> MAQYYPGTTKVAQNRRNFCNPEYELEKLREISDEDVVKILGHRAPGEEYPSVHPPLEEMDEPEDAIREMVEPIDGAKAGDRVRYIQFTDSMYFAPAQPYVRSRAYLCRYRGADAGTLSGRQIIETRERDLEKIS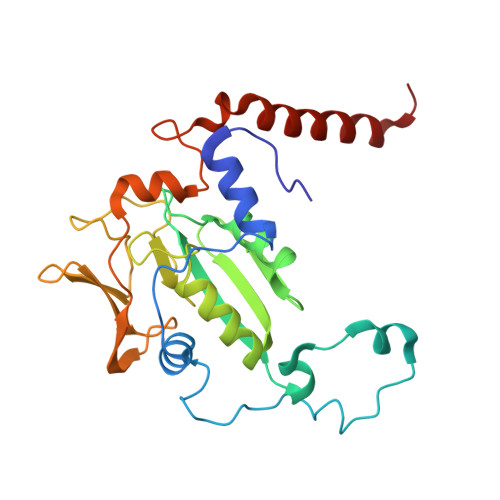KELLETEFFDPARSGVRGKSVHGHSLRLDEDGMMFDMLRRQIYNKDTGRVEMVKNQIGDELDEPVDLGEPLDEETLMEKTTIYRVDGEAYRDDVEAVEIMQRIHVLRSQGGFNLE>MEGKVYHFRVKFGDTDAAGIVFYPNYYKWMDEACHHFLTELGFPTSELIDKKIGFPIVEATCQFKAPLLFADHVFIRTSIRELKDKSFILEHHFIKQGRVIASGHEKRVWANFSNGKLAVCPIPSSVRVAFANI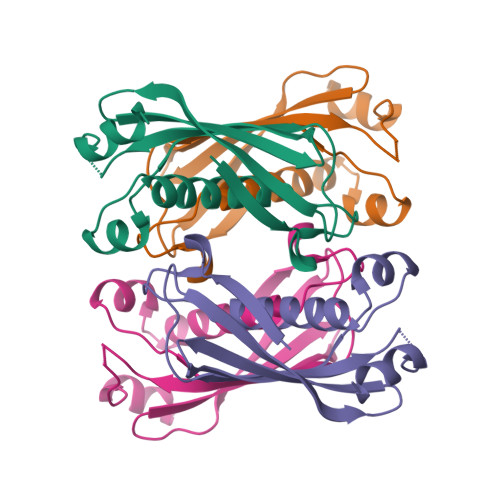GTCE[4x]> MDILENYVSFDEQARDINIAFDKLFGRDDISHMNNFSINKRSYYNCLDQISDDLNLVLNKYNDLAYSLLEIRYNMATKENYTHMEFYSDIERLFIKNEKLLNVISDIVEEEYDLDLNQASKGKKINIELQVTDNLNKIYLKSSVLMRILIPILCDFNCDDDINEVLVYDIFKEVIKSFDDGKKNALNKLYKIIYSRVFETKYSDVVIWTYLKNMSTDLMIIVKDYFKVIIKKIFPKLKHNSSVISYLDVVIKQKLKYLFTFKYPISYKPLKAETTDDEELSEQERMEINLLRNDQGNSIINECSIKQEIAKIKKKYNVTDEVMKEFINGRELNSIQIYLVKIYYSNKFKVNSNKNDIFYLLYGMTRELGEMNFSIIPEILSCAIAPNVRKMNNRKKLVDKIIHSDKYSYLLKSYLPIKNILDKNNVILQLMTIKNAKFMNKENKEVDFSTDHLAEEVLDMLLCI;> MDDISVIKNEDYEGSHRFLAEELLMPNANKTDGNRSTMFCSHLAQAVTLQKAEPPLVYTNFENQVGKYSTAGYRKANSNYKVIEKIYKNDYNYVLIVQDQETGEYTLFERAECEFLTEHYGFQWDNDKIDSLKKDDTIEKDTVLYKNTCYDENMNFGYGVNLNAAYFSYKNETLEDAIVISESAAKKLGTFSVNKVKVSVNTNDILLNLYGDNENYKGFPDIGEHIKNQIIASRRRFDYNTALYELKNLNEMRDSDTPFFADGKIVDIEIFSNVPEEELKVQKYNEQVLYYINKQKEFSNNVYQKLKKIVEGKDNNVSDKLLHFYNNCKMRID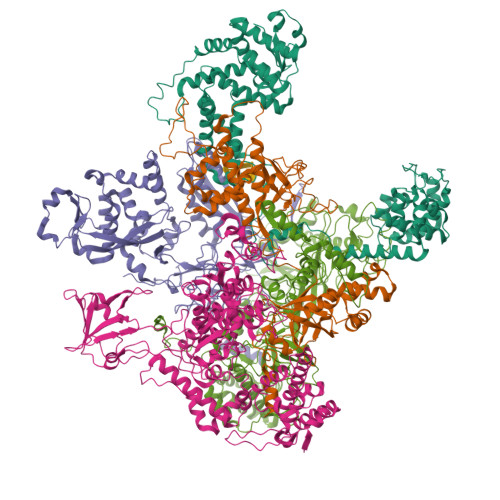ENISYTYQNSKFSGFIMEFTILEEEPLNKGSKITGRYGNKGVISKILPDDQMPTVAEGRFKGLKADICLNPLGVFNRLNPSQLIEQELNWIAKFIRKDMEEAGSNEEKVSILLDFLNRVNKEETELMEEFINSLNKTELEEFLNDIIENGIPICQKPFFGNIGLDELWELYNHYDHIDYFKCEGISTPLIIGEIYMVRLKHEPHSKFSARSTSFMNLRGLPAKSKNFKEHKDLYSKTPVRIGNMEISNLSLTNEMGSIMDMLNSYSNNETNRRELIMQLLTGNPFDTNIDLSDVESGTSKILKSLFTCLGLSIDDVEEEWENKLNGKVEDEK;> MEKTYNLNDILLSNEYEKIKEDIKEEIINDMASKKVKYSNTSEFAKNDFLKDEFIDLVVDGETYEITYGNLITLLIVARPFNHFKVPMTEDLLFDLSDLKEYQNYYTTLLEHFGYSNEIKSIIKDVISELAIFSGDINVTFGNTVSIKSLIDLGNKVKRFRELLHYRLPNDEALEFNDIEAIIKKNLDEIMKILSETDNMLRYYIDSGAGINSKQFGQVLSLVGSKPDLFGKIIPYPINTSFLRGLDVRSFYINALGARKALITNYQQVRNSGYLTRKISMLLMDTKLIDLDDCGSHENNYLSINVENKDVLKRFSKRSYLNNNGELVEIDINDESLIGQVIKIPSPTTCASNEGVCRKCYGKLFDINKDLNIGMIAVLLLTDPLTQRLLSAKHLLETRSSKIDWGTNFEENFIVNRNLIYPKVYNGTVIIKEDDFKEDEETEEQVFDTFTLKSGNRFISISSPMRLFLNKDLKKQLDESFYNIEEMQFEIPLNKLDEGDSFATFIMDNNELSKPLREIKDLIETNKYIKDHNVNEVVNYFIYLLNESGINIQSVHSELIIREMMKLDDSDRTQFKNDKMPDYEIFRITDANLKGDSLSRSLLFEQVKKQLTTLDYDTFNKTKSSILDKLL;> MISNFRKFHGNKNQEKFNENLILNKENESILNYLDPICKTLEIIPEITYLGSSVEPINKVYKFNKEEKTSDIERSELQLIKMSFLIEKDDKKEEINKFIYFPKLIDSQYFIINGNRYYPIYQLLDSGTYRTNKALTLKTLLMPIVLREKKETFDDINGETHTMLNVDLDLFKSKVPFLIYFFSKFGFEGTLEYFGLQDLIHVLMKEDLDQLDEDEINDNVIFMITKNISLVVDKNFFSNKNNQIIIATLLNCFNTRIKIDKIYEKDYWVKKLGGYFTTNNSNKQEKGEGIILSFERILDEWTKKILRTEEKNKEDIYSVVRWMINNYLALVKQDNMNLANKRIRLYEYLLHPLLIKFSKGTYRVLNNRNSNKFEKIKTIFSNIQEGFLVKKIINNELLRYDNSVNSISLFTLILRYTQSGPQSPFSSNSTNNKLRGLHPSYLGRLGLTSTSAGDPGASGSLTPFLELPENSYMHFTEEPEINLNIDDISIDEVIES;> MGSSHHHHHHSSGENLYFQGHHMGKKLSLIDFNEIYNEENLITRANPIENHEFSDDGIYSERIFGSYNEDDDDKDIDTIGWINIEPYYIINPILFTIIKKCIPSINKIINYQQSIDQNGENIDLTEEIGEDDYIGLVKFKDNFDDLLEKYTDKKKYQKEYDFLIENHDKIFINKLPVFSHKLRPATLLTGSKGKVLAFDEINNYYNFVIEYINQINEGVVSDDSIDLLLLPLLYNMQFYANNILTRIISEYLRGKKGFLRKNIMGSRINFSARNVITPLIGHPIDEVAMPYKTFAELYKFQLINLISKVKGINYNEALKFWEKGILGFNQELYNYMEELITKTKGGCTFLLNRNPTISIGSILYLKIGLIKKDYKDLTLGISNNLLSALSGDYDGDVLNIIPVFDNKMKEHFSLLSPQNFLVDRNNGRFNGDFDLQKDQILGIFILNN GlgE is an α-maltose 1-phosphate:(1→4)-α-d-glucan 4-α-d-maltosyltransferase (starch synthase (maltosyl-transferring), EC 2.4.99.16) and a member of the carbohydrate-active enzymes database (CAZy) GH13_3 family. It is the third and defining enzyme of the four-step GlgE pathway that is responsible for the biosynthesis of a branched α-glucan. The key contribution that GlgE makes is to preferentially extend A chains, limiting the opportunity for GlgB to introduce a second branch into B and C chains. The enzyme consists of five domains, four of which are typical of the α-amylase family.

To prevent GlgE from catalyzing such reactions, a D394A GlgE variant that lacks the nucleophilic side chain was generated. This GlgE variant was co-crystallized with a preparation of maltodextrin, which contains a wide range of both linear and α-1,6 branched oligosaccharides according to mass spectrometry and NMR spectroscopy. However, a linear malto-oligosaccharide was observed bound to the cyclodextrin binding site for the first time. Five sugar residues were resolved, four of which occupied very similar positions to those observed with β-cyclodextrin such that they interacted with Trp-448 and Arg-449. Similarly, another oligosaccharide was observed in the structure of the D394A GlgE variant obtained with maltodextrin. Again, five glucose residues of an α-1,4-linked malto-oligosaccharide were wrapped around the side chain of Tyr-646 with the reducing end glucose residue being flipped relative to the others. Remarkably, several additional glucose residues were resolvable within the electron density. In one copy of the GlgE subunit within the crystal, an additional four sugar residues were present that made no direct contact with this subunit but instead interacted with a subunit from a neighboring GlgE homodimer in the crystal lattice. There was an α-1,6 linkage between the reducing end of the proximal pentasaccharide and the second residue from the reducing end of the distal tetra-saccharide. Therefore, the protein-bound pentasaccharide constitutes an A chain emanating from a tetrasaccharide C chain.

>MGSSHHHHHHSSGLVPRGSHMPATHHSSATSAERPTVVGRIPVLDVRPVVQRGRRPAKAVTGESFEVSATVFREGHDAVGANVVLRDPRGRPGPWTPMRELAPGTDRWGATVTAGETGTWSYTVEAWGDPVTTWRHHARIKIPAGLDTDLVLEEGARLYERAAADVPGREDRRELLAAVDALRDESRPAASRLAAALTPQVDAVLARHPLRDLVTSSDPLPLLVERERALYGAWYEFFPRSEGTPHTPHGTFRTAARRLPAIAAMGFDVVYLPPIHPIGTTHRKGRNNTLSATGDDVGVPWAIGSPEGGHDSIHPALGTLDDFDHFVTEAGKLGLEIALDFALQCSPDHPWVHKHPEWFHHRPDGTIAHAENPPKKYQDIYPIAFDADPDGLATETVRILRHWMDHGVRIFRVANPHTKPVAFWERVIADINGTDPDVIFLAEAFTRPAMMATLAQIGFQQSYTYFTWRNTKQELTEYLTELSGEAASYMRPNFFANTPDILHAYLQHGGRPAFEVRAVLAATLSPTWGIYSGYELCENTPLREGSEEYLDSEKYQLKPRDWTRAAREGTTIAPLVTRLNTIRRENPALRQLRDLHFHPTDKEEVIAYSKRQGSNTVLVVVNLDPRHTQEATVSLDMPQLGLDWHESVPVRDELTGETYHWGRANYVRLEPGRTPAHVCTVLRPSHPQIGGSHTT[2x]>MTKPLDGINVLDFTHVQAGPACTQMMGFLGANVIKIERRGSGDMTRGWLQDKPNVDSLYFTMFNCNKRSIELDMKTPEGKELLEQMIKKADVMVENFGPGALDRMGFTWEYIQELNPRVILASVKGYAEGHANEHLKVYENVAQCSGGAAATTGFWDGPPTVSGAALGDSNSGMHLMIGILAALEIRHKTGRGQKVAVAMQDAVLNLVRIKLRDQQRLERTGILAEYPQAQPNFAFDRDGNPLSFDNITSVPRGGNAGGGGQPGWMLKCKGWETDADSYVYFTIAANMWPQICDMIDKPEWKDDPAYNTFEGRVDKLMDIFSFIETKFADKDKFEVTEWAAQYGIPCGPVMSMKELAHDPSLQKVGTVVEVVDEIRGNHLTVGAPFKFSGFQPEITRAPLLGEHTDEVLKELGLDDAKIKELHAKQVV[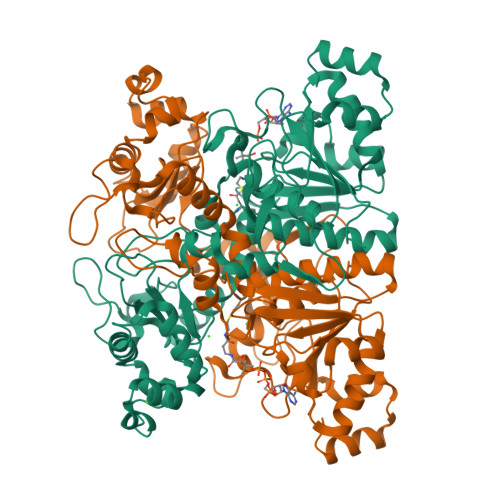2x]>MHHHHHHSTATNPLDLDVCAREPIHIPGLIQPYGVLLVIDPADGRIVQASTTAADLLGVPMAALLGMPYTQVLTLPEAQPFAVDDQPQHLMHAEVRFPQRATPPASAWVAAWHLYPQQWLVEMEPRDARLLDVTLREAMPLLRSVERDPGIAEAAVRVAKGLRSLIGFDRVMIYRFDEEWNGDIIAEARKPELEAYLGLHYPASDIPAQARALYLRNRVRQIADVGYQPSPIQPTVHPQLGTPVDLSDVSLRSVSPVHLEYLANMGVTATLVASIVVNDALWGLISCHHYSPHFTN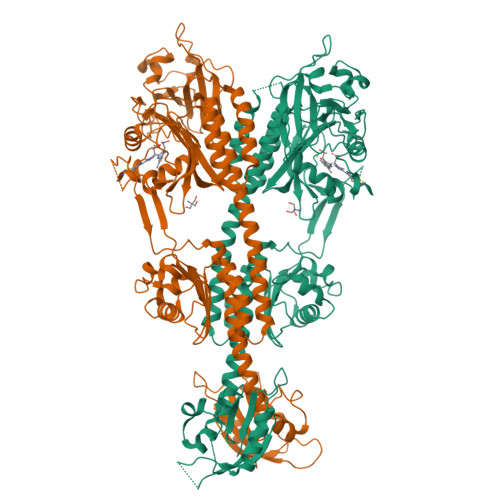HAMRDVTDAVARTLAGRIGALQAVARARLESVLLTVREKLITDFNDAEHMTVELLDDMAPDLMDVVDADGVAIFHGNDISRHGTTPDVAALRRIRDHIESEHHEALREDAVGALHVDAIGEVFPELADLAPLAAGFIFVPLMPQSRSALLWTRREQIQQIKWAGNPQLAKLEDIPNSRLSPRKSFDLWQQTVRGRARRWSPLHLESARSLRVLIELMERKRFQQDFTLLEASLSRLRDGVAIIERGTANAAHRLLFVNTAFADVCGSDVAELIGRELQTLYASDAPRANVELLQDALRNGRAAYVTLPLQVSDGAPVYRQFHLEPLPSPSGVTAHWLLQLRDPE[2x]>[2x]QGNDTSEVMLLDTGWEFSQSGTEKWMPATVPGTVHQDLISHELLPNPFYGMNEKKIQWVENEDWEYRTSFIVSEEQLNRDGIQLIFEGLDTYADVYLNGSLLL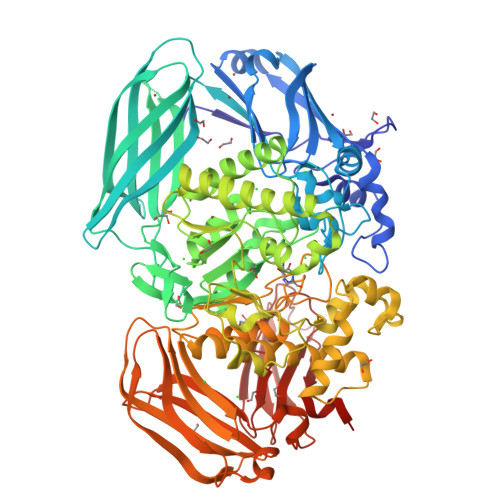KADNMFVGYTLPVKSVLRKGENHLYIYFHSPIRQTLPQYASNGFNYPADNDHHEKHLSVFSRKAPYSYGWDWGIRMVTSGVWRPVTLRFYDIATISDYYVRQLSLTDENARLSNELIVNQIVPQKIPAEVRVNVSLNGTTVTEVKQQVTLQPGINHITLPAEVTNPVRWMPNGWGTPTLYDFSAQIACGDRIVAEQSHRIGLRTIRVVNEKDKDGESFYFEVNGIPMFAKGANYIPQDALLPNVTTERYQTLFRDMKEANMNMVRIWGGGTYENNLFYDLADENGILVWQDFMFACTPYPSDPTFLKRVEAEAVYNIRRLRNHASLAMWCGNNEILEALKYWGFEKKFTPEVYQGLMHGYDKLFRELLPSTVKEFDSDRFYVHSSPYLANWGRPESWGTGDSHNWGVWYGKKPFESLDTDLPRFMSEFGFQSFPEMKTIAAFAAPEDYQIESEVMNAHQKSSIGNSLIRTYMERDYIIPESFEDFVYVGLVLQGQGMRHGLEAHRRNRPYCMGTLYWQLNDSWPVVSWSSIDYYGNWKALHYQAKRAFAPVLINPIQQNDSLSVYLISDRLDTMEQMTLEMKVVDFDGKTLGKKIQVHSLEVPANTSKCVYRAKLDGWLTPEDCRRSFLKLILKDKSGHQVAESVHFFRKTKDLQLPPTSVSYQMKQTDGKCELTLFSSMLAKDIFIETPLQGARYSDNFFDLLPGERKKVIITSPRIKKGEELPVNIKHIRETYKEHHHHHH>HMASMKKKGSVVIVGRINLSGDTAYAQQTRGEEGCQETSQTGRDKNQVEGEVQIVSTATQTFLATSINGVLWTVYHGAGTRTIASPKGPVT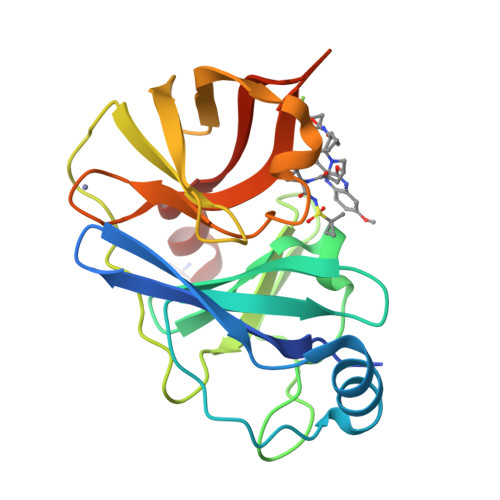QMYTNVDKDLVGWQAPQGSRSLTPCTCGSSDLYLVTRHADVIPVRRRGDSRGSLLSPRPISYLKGSSGGPLLCPAGHAVGIFRAAVSTRGVAKAVAFIPVESLETTMRS[2x]> DDKAMAGNFWQSSHYLQWILDKQDLLKERQKDLKFLSEEEYWKLQIFFTNVIQALGEHLKLRQQVIATA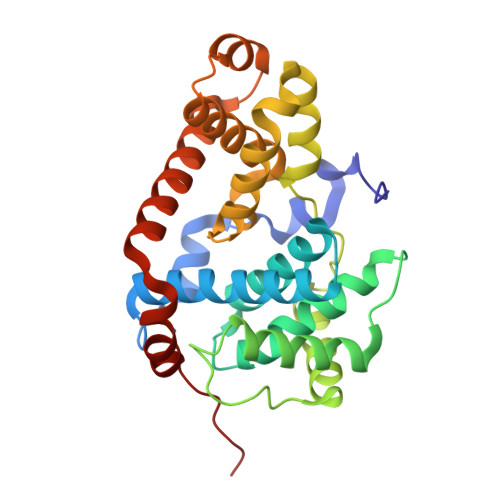TVYFKRFYARYSLKSIDPVLMAPTCVFLASKVEEFGVVSNTRLIAAATSVLKTRFSYAFPKEFPYRMNHILECEFYLLELMDCCLIVYHPYRPLLQYVQDMGQEDMLLPLAWRIVNDTYRTDLCLLYPPFMIALACLHVACVVQQKDARQWFAELSVDMEKILEIIRVILKLYEQWKNFDERKEMATILSKMPKPKPPP> SNAMKVKIYTRNGCPYCVWAKQWFEENNIAFDETIIDDYAQRSKFYDEMNQSGKVIFPISTVP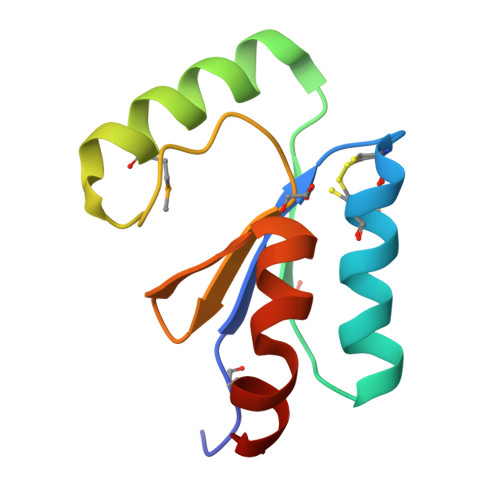QIFIDDEHIGGFTELKANADKILNKK>[2x]MAPMSEKQLADVVERTVTPLMKAQAIPGMAVAVIYQGQPHYFTFGKADVAANKPVTPQTLFELGSVSKT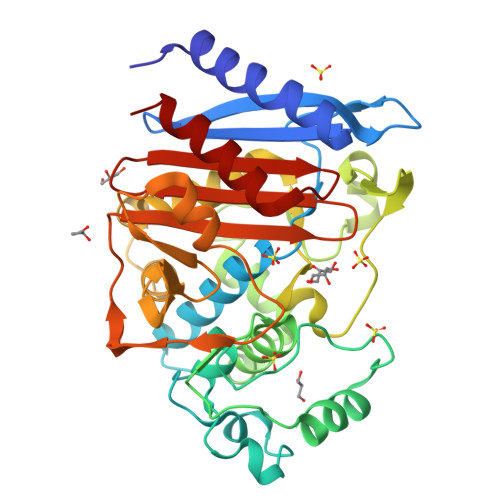FTGVLGGDAIARKEISLADPVTKYWPELTGKQWQGIRLLDLATYTAGGLPLQVPDNVTDNASLLRFYQSWQPKWAPGTTRLYANTSIGLFGSLAVKPSGMRFEQAMAERVFKPLKLNHTWINVPHAEESHYAWGYREGKAVHVSPGMLDAEAYGVKSNVKDMASWVMANMAPETLPPSTLQQGIALAQSRYWRVGAMYQGLGWEMLNWPVDVKTVVDGSDNKVALVPVAEVNPPAPPVKASWVHKTGSTGGFGSYVAFIPEKQIGIVMLANKSYPNPVRVETAYRILETLQ>MAMKREQTIENLYQLAQLTQQVQADRIEIVLEERRDEHFPPMSKALMETRSGLTRRKLDEAIAKMEEAGHQFTKNNANHYSISLSEAHMLMDAAGVPKFHERKKNNENKPWIINVQNQKGGTGKSMTAVHLAACLALNLDKRYRICLIDLDPQGSLRLFLNPQISLAEHTNIYSAVDIMLDNVPDGVQVDTEFLRKNVMLPTQYPNLKTISAFPEDAMFNAEAWQYLSQNQSLDIVRLLKEKLIDKIASDFDIIMIDTGPHVDPLVWNAMYASNALLIPCAAKRLDWA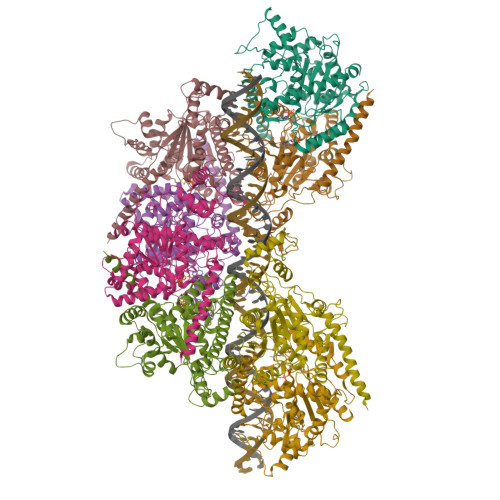STVNFFQHLPTVYEMFPEDWKGLEFVRLMPTMFEDDNKKQVSVLTEMNYLLGDQVMMATIPRSRAFETCADTYSTVFDLTVNDFEGGKKTLATAQDAVQKSALELERVLHSHWSSLNQG[8x]> MAGALRLVLGDQLSDNLSALVDADLSRDQVLMVESRVEATAWKHHKQALVLVWSAMRQFAERLRARGFNVRYVTLEDPDNTGSIGGELRRALEARAFDRVIRTACGKWGLESHLLSLDLPVPMETREDDRFLCSRAQFAAWAEGRRELRMEFFYREMRRKTGLLMDGDQPAGGRWNFDAENRRKLPPGLRPPERLRIPPNPTTQTVLEQVSRGFDDHFGEVEGFGWPTNPDEATAILDHFIADMLPSFGDWQDAMSWRRPFLWHSLISPALNIGLLDPLDICRRAEAAWREGRAPLNAVEGFIRQIIGWREFVRGIYWLKMPEYAQRNALDAQGKLPGFYWTGQTDMACVADTVRAAHDHAYAHHIQRLMVTGNLAMLLGVHPDAVDDWYMVVFADAYEWVEMPNTRGMATFADGGIVGSKPYAASGAYIDRMSDYCKGCRYDVKKRLGDDACPFNALYWDFIDRHAQRLAGNGRMMMPLRTLEKMPDAEREAFRKQARALRVKMGVSG

Photolyases repair UV damage to DNA by using absorbed blue light. Within the photolyase/cryptochrome superfamily (PCSf), a major subgroup consists of prokaryotic (6–4) photolyases. These enzymes rely on flavin adenine dinucleotide (FAD) as a catalytic cofactor, besides an ancillary antenna chromophore, and a [4Fe-4S] cluster with yet unknown function. For the prokaryotic 6–4 photolyase of Caulobacter crescentus, we investigated structural changes associated with its different redox states by damage-free crystallography using X-ray free-electron lasers.

The side chain of K48 is almost halfway located between the DLZ antenna in the N-terminal domain and the FAD’s isoalloxazine. Although the displacement of the K48 side chain may be dictated by the changed electrostatics around the isoalloxazine moiety and Wat1 movement, this residue participates in the stabilization of DLZ binding. A K48A mutation results in a partial loss of the DLZ antenna, which can be observed through UV/vis spectroscopy. This is further supported by the structure of the K48A mutant, where the DLZ antenna appears to be only partially occupied. In the 1.5 Å structure of the K48A, we find only an occupancy of ∼50% for the antenna.5-(3-ethoxyphenyl)-1,3,4-thiadiazol-2-amine | C10 H11 N3 O S | 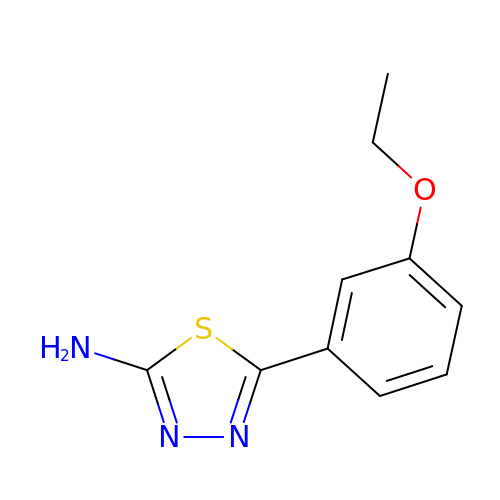APEORNRUGDLVDP-UHFFFAOYSA-N> MMRGIDSRHELDPTLLLRDTRTFTQRLADFFADPTNISIVLISLAAVSYYFSEAATFLLIMGGIFFLYSYTRKQKLPFRLPQISRAKDYNDLKPGINKPNIARGITFFGNDRKTGEELWFANDDMRTHALIFGSTGSGKTETLVSLSYNALVQGSGFIYVDGKGDNSLYAKVFSMVRSMGREDDLLLINFMTGARDIVGPQEKRLSNTLNPFCQGSSSMLTQLVVSLMGSSGQSSDGDMWKGRAIAFVEALMRLLVYMRDEGAILLDANTIRNYFDLQRLESIVIDKVFPRDDQESVNIETIPKLVTDPLRNYLNTLPGYNKEKKGKQVSQVLEQHGFITMQLVRSFSSLADTYGHIIRTNLAEVDFKDVVLNRRILVVLLPALEKSPDELSNLGKIIVSSLKAMMAAGLGEEVEGDYRDVILRKPTNAPTPYMCILDEYGYYAVQGFAVVPAQARSLGFSAIFAGQDLPAFQKASKEEAASIGANTNIKICMKLEDPTETWDFFTKTAGEAYVTKVDSFQTKETSIANSYMDTKSSSFEKRARVDLLDLKEQTEGEAHIFFKSKIVRARMFYANPKPVKQLKINQFLKVEPPPDDYLMKLQKQLASFQSILESGDLSINKAVENEEITLISKALKESTIVEPIERGVAALIAFHGQNEPEPVEDIVEEEVEGALTIFSKLRIDPNAPPILVADKEVFSEPLLPINETRNQMITIERLAGAKDKYAGTVANELIKDFQIATSYPPEERDVIDVQELTGIIRDLSAKISAEREKANKKAAEELT;> MYIEMAQQQQQSGSDNSMAPVWIVILLFITAYFVWALAHQYIVSFVFTINIWQARLVNLFLNNQLLANQIYLMQTLDPNTVNWDQMVTVMRAVGDYMRYPVICILVVLAFVLYNSNVTLKYRKTYDMKSLRAQEQFNWPAIMPIVKEDLVSQDVNKGPWAMALTPMEFARKYNLLRKDDALLDNPVPGEEMTAGIRRGDAKRVFTMQLGPYWDGFERCSPQAYALSAVFMARMNRDRDAANNILKVLDKTFVDGKPDFSVARPVMKKYQNSELVQEVVAKHAYVLTVIASLLEAAREDGVVPSSEFLWLKPVDRRLWYMLNCVGRQTPYSEVAGPFAHWKAEKEMGRRSLVPMIDEAIRALEIAVKEVRLTPRQMEELEP;> MADNQQRCELKLIASPGSWRLYSARKIDERFKSYEQKIFQRDRYTCQFCGFQARLYQDIVNLDGDYTNNRLSNLVTACCFCAQCFFVESVGVGGYGGGTLIYLPELTQAELNSLCHVLFCAITNDTGYKSSAQNIYRSFKFRSQIVEEKFGEGTSDPAIFGQLMIDSGVNSEEIREKLFKNIRLLPSRAKFRKQIEKWAASALEEIAD;> MDEIKKDDELSQWLSTYGTITAERILGRYNISLPQDEILEAINIPSSFYRHLLQIPLKNVLNGIVIQQASDYHVYAQKLLIDYLLSGESSKEPDSQGAGTRESLEDERQR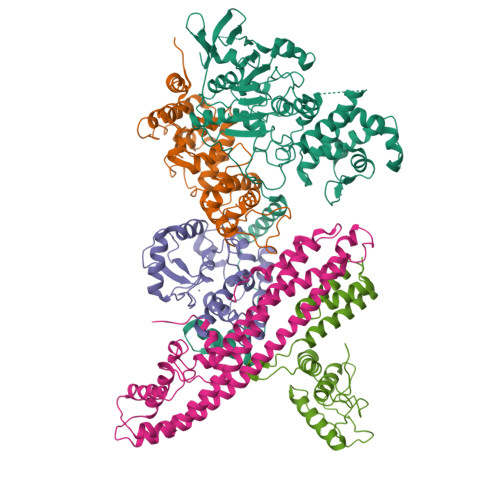LVQLGDEFHKLELEQDNLIASSQASLMKISIDWNTKLETTLSKLNSLYKNTNSKIKKNAIRKALIKAFIHCDLVKDQSQKNKYQLIDKLNQTLAVSVGAELKESILTNLSELFQILEALNTKLDEFTDRTNHLSQQAKSFRTQFYEVILRIIELIKLLPEYKIDPAQDAINREPLYFDRTIGER;> MPKYTLPTRDALLKAMQVGETSIEAAEYMATRFEQILTKAKLLPECNDMLEKIKEYAQFVKFKLLSSAQVWSGQERPTSDYQNTQENKAEFLASHLEGLPSGLKLEVAIGDDAKILRGFSSNGKMVEGDQLKTMDGLLEGWLAKNSLAISGGAVVKIDNTGNQTKVDPQEIRQLINDSEKGVAKYFADKGVGMEVAQRTYQEPKALETKREEIRQEIESGAEAPTTQSIR>GPGMKDCSNGCSAECTGEGGSKEVVGTFKAKDLIVTPATILKEKPDPNNLVFGTVFTDHMLTVEWSSEFGWEKPHIKPLQNLSLHPGSSALHYAVELFEGLKAFRGVDNKIRLFQPNLNMDRMYRSAVRATLPVFDKEELLECIQQLVKLDQEWVPYSTSASLYIRPTFIGTEPSLGVKKPTKALLFVLLSPVGPYFSSGTFNPVSLWANPKYVRAWKGGTGDCKMGGNYGSSLFAQCEAVDNGCQQVLWLYGEDHQITEVGTMNLFLYWINEDGEEELATPPLDGIILPGVTRRCILDLAHQWGEFKVSERYLTM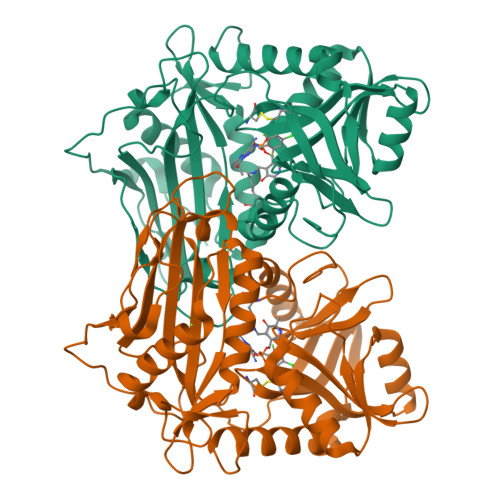DDLTTALEGNRVREMFGSGTACVVCPVSDILYKGETIHIPTMENGPKLASRILSKLTDIQYGREERDWTIVLS[2x]Crocagins (1 and 2)24 are very small, intriguing RiPPs that possess a tetracyclic ring system, which consists of a pyrroloindoline fused to a tetrahydropyrimidinone moiety. Here we use in vitro experiments to demonstrate that three proteins, CgnB, CgnC and CgnE, are sufficient for the production of the hallmark tetracyclic crocagin core from the precursor peptide CgnA. We further show that the hydrolase CgnD liberates the crocagin core scaffold, which is subsequently N-methylated by CgnL. The crystal structures of the homologues CgnB and CgnE reveal them to be the founding members of a peptide-binding protein family and allow us to rationalize their distinct functions.

We hoped that the crystal structure of CgnD might yield additional insights and determined the structure to 2.35 Å resolution. Intriguingly, it appeared as if the dimer provides two antiparallel channels for substrate binding that terminated at the respective active sites. The catalytic triad comprised Asp325, His328 and Ser79, and the distance observed between the Asp325 atom Oδ2 and His328 atom Hδ2 was within the expected range (1.8 Å). The distance between His328 atom Nε2 and Ser79 atom Hγ could not be determined because a sulfate ion was bound at the active site, which led to a rotation of the Ser side chain. Removal of the sulfate in silico and subsequent rotation of the Ser side chain did not allow the distance to decrease below 2.8 Å. The resulting lack of nucleophilicity appeared a probable cause for the slow turnover and was supported by our inability to label CgnD with phenylmethylsulfonyl fluoride. When CgnD was added to the product of CgnA–CgnB–CgnC–CgnE reactions containing 3a and 3b, we observed the slow production of 4a ([M]+ calculated, 495.2238; observed, 495.2239; mass error (Δ) = 0.2 ppm), which represents the crocagin core scaffold (des-methyl and des-carbamoyl) and also corresponds to the mass produced by the cgnE knockout. Slow proteolytic processing of modified precursor peptides has been observed in a number of RiPP biosynthetic pathways and may be linked to biosynthetic timing. The intermediates 3a and 3b are then cleaved by CgnD to release the core scaffold and make the N terminus available for methylation by CgnL.

>[2x]GAMASTTLETRDELTPQMKEYDRAGRVWVPYLNYFHRPNHRSPVVNTDSRGFRFVVGKDGRTFSEFEREPGERVRALVGGSTVFGVGATGDAATLPSLLSQRGPARWLNFGGRAFSSTQELMLFLFHARSLGALEKVTLLSGVNNLLLFYLSRDYAKDYGSFFATEVRRAFAGDAPSPAKSGVIGRLKSIAGGRRAKVEAPEPEIVLPIVDHDAQKTDLLHAIERDLSTWKLLSGALQFELCYVLQPLAGWVRKKPSPEETRLFADLDDQQGEAWRQILREKMDLAQYAWFSKSLADICRTQEIPFLDMNATLSALDLDGRWIFVDRVHLTDEGNEVLTQALVEGGAT>ATMALKTVDAKQTTSVCCYCSVGCGLIVHTDKKTNRAINVEGDPDHPINEGSLCAKGASTWQLAENERRPANPLYRAPGSDQWEEKSWDWMLDTIAERVAKTREATFVTKNAKGQVVNRCDGIASVGSAAMDNEECWIYQAWLRSLGLFYIEHQARIUHSATVAALAESYGRGAMTNHWIDLKNSDVILMMGSNPAENHPISFKWVMRAKDKGATLIHVDPRYTRTSTKCDLYAPLRSGSDIAFLNGMTKYILEKELYFKDYVVNYTNASFIVGEGFAFEEGLFAGYNKETRKYDKSKWGFERDENGNPKRDETLKHPRCVFQIMKKHYERYDLDKISAICGTPKELILKVYDAYCATGKPDKAGTIMYAMGWTQHTVGVQNIRAMSINQLLLGNIGVAGGGVNALRGEANVQGSTDHGLLMHIYPGYLGTARASIPTYEEYTKKFTPVSKD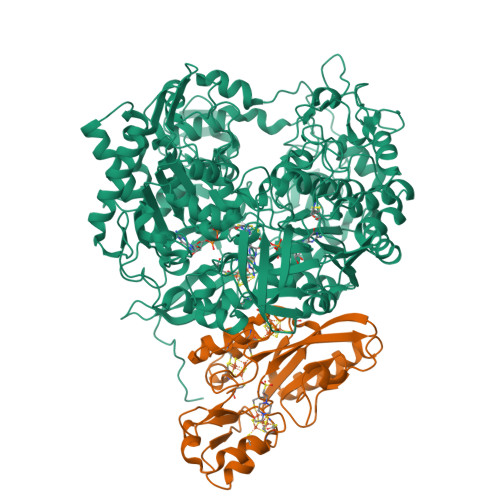PQSANWWSNFPKYSASYIKSMWPDADLNEAYGYLPKGEDGKDYSWLTLFDDMFQGKIKGFFAWGQNPACSGANSNKTREALTKLDWMVNVNIFDNETGSFWRGPDMDPKKIKTEVFFLPCAVAIEKEGSISNSGRWMQWRYVGPEPRKNAIPDGDLIVELAKRVQKLLAKTPGKLAAPVTKLKTDYWVNDHGHFDPHKIAKLINGFALKDFKVGDVEYKAGQQIATFGHLQADGSTTSGCWIYTGSYTEKGNMAARRDKTQTDMQAKIGLYPGWTWAWPVNRRIIYNRASVDLNGKPYAPEKAVVEWNAAEKKWVGDVPDGPWPPQADKEKGKRAFIMKPEGYAYLYGPGREDGPLPEYYEPMECPVIEHPFSKTLHNPTALHFATEEKAVCDPRYPFICSTYRVTEHWQTGLMTRNTPWLLEAEPQMFCEMSEELATLRGIKNGDKVILESVRGKLWAKAIITKRIKPFAIQGQQVHMVGIPWHYGWSFPKNGGDAANILTPSVGNPNTGIPETKAFMVNVTKA[2x];>[2x]SKGFFVDTTRCTACRGCQVACKQWHGNPATPTENTGFHQNPPDFNFHTYKLVRMHEQEIDGRIDWLFFPDQCRHCIAPPCKATADMEDESAIIHDDATGCVLFTPKTKDLEDYESVISACPYDVPRKVAESNQMAKCDMCIDRITNGLRPACVTSCPTGAMNFGDLSEMEAMASARLAEIKAAYSDAKLCDPDDVRVIFLTAHNPKLYHEYAVA>[2x]MSISISYSTTYSGWTVADYLADWSAYFGDVNARPGQVVDGSNTGGFNPGP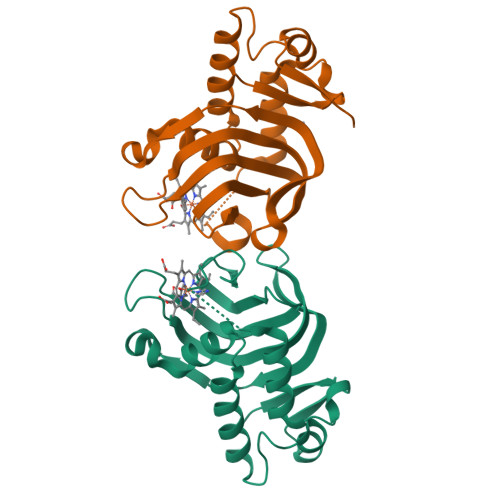FDGSQYALKSTASDAAFIAGGDLHYTLFSNPSHTLWGKLDSIALGDTLTGGASSGGYALDSQEVSFSNLGLDSPIAQGRDGTVHKVVYGLMSGDSSALQGQIDALLKAVDPSLSINSTFDQLAAAGVAHATPAA> TLTVHVRSEEWDLMTFDANPYDSVKKIKEHVRSKTKVPVQDQVLLLGSKILKPR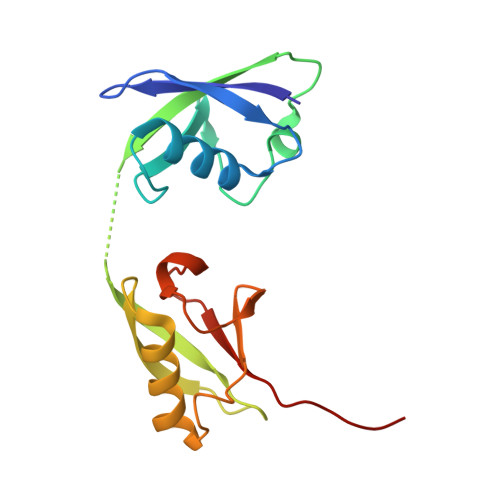RSLSSYGIDKEKTIHLTLKVVKPSDEELPLFLVESGDEAKRHLLQVRRSSSVAQVKAMIETKTGIIPETQIVTLNGKRLEDGKMMADYGIRKGNLLFLASYSIGG> MQWQELYRQRVCSADEAVVDSLKPGTKVVFGHAAAAPVRFSQAMYRQREKLENITVFHMLYFGDAPHLAPEMRSHVHPTLNFLEGNSRPASRDRRVDFIPCHFHEVPELFRQGFFPLDVAVVQVSTPNEE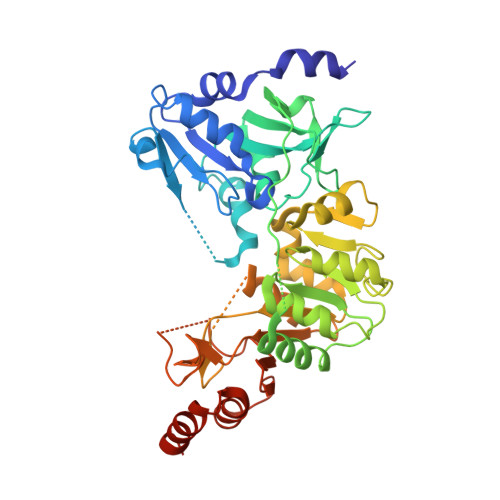GYCSFGVSCDYTKAAAECAPVVVAEVNKQMPFIGGENLIHISKLTHIIEVDEPIAEVLPPAGSDLELRIGQNCASLIKDGDTLQLGIGGIPDAVLRALEGHKDLGIHTEMFTDGVMRMIRKGIINGKKKTLHPEKVVTSLIFGSKELYDFVNNNPVIECYPVDYINNPDVIGKNDRMVSINSCLEMDLMGQAASESIGYEQFSGSGGQVDFLRGAKRSKGGISIMAFPSTAKKGTESRIVPILKEGACVTTGRNEVDYVVTEYGVARLRGATLRQRAEALTAIAHPDFRPALEEEIRRRFELEHHHHHH> MVIVPEGTQLDEKQHIVINNGAEPQSFDPHKTEGVPESNVAYQLLEGLVTSDSEGKLQPGAAESWENTPDFKTWTFHLRKDAKWSNGDPVTAHDFVFAWRRLVDPATAAPYASYLSYLQVENAQDIIDGKKKPAELGVEAKDDYTFVVHATNPVPYAVSLTTHQSLLPLPQKVVEKLGDAWVKKENYVGNGAYKLANHIINEKIEFERNPLYWNDKETVINSATFLAIENPSTDVARYRAGDLDMTSYGLPPEQFAKLKKELLGEVYVTRTLGTYSYELNNKK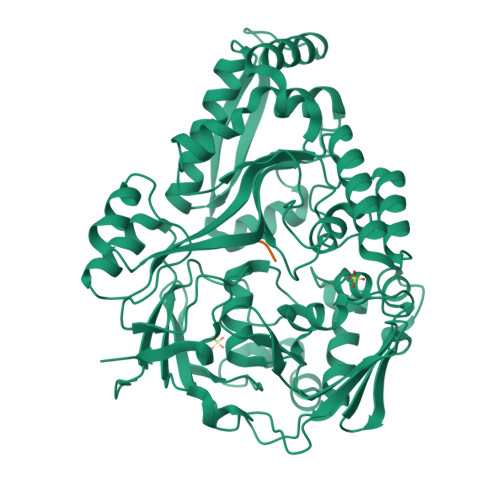APFDNVNIRKALNLSLDRNVITDKVLGQGQTPTYVFTPTYIEEGHLIQQPAYSKEPMAQRNEEAIKLLEEAGYSKANPLKFSILYNTNENHKKVAIAAASMWKANTKGLIDVKLENQEWKTYIDSRRAGRYDVARAGWHADYNQATTFGNYFLSNSSNNTAKYANPEYDKAMAESYAATDAEGRAKAYAKAEEILGKDYGIVPIFNYVNPRLVKPYVKGYSGKDPQDHIYLRNLYIIKHLEHHHHHH;> KKK>TLVKDILSKPPITAHSNISIMEAAKILIKHNINHLPIVDEHGKLVGIITSWDIAKALAQNKKTIEEIMTRNVITAHEDEPVDHVAIKMSKYNISGVPVVDDYRRVVGIVTSEDISRLFGGK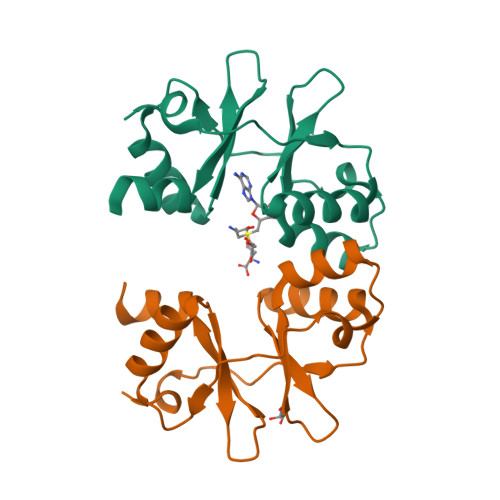K[4x]>[2x]TDTTLPPDDSLDRIEPVDIEQEMQRSYIDYAMSVIVGRALPEVRDGLKPVHRRVLYAMFDSGFRPDRSHAKSARSVAETMGNYHPHGDSSIYDSLVRMAQPWSLRYPLVDGQGNFGSPGNDPPAAMRYTEARLTPLAMEMLREIDEETVDFIPNYDGRVQEPTVLPSRFPNLLANGSGGIAVGMATNIPPHNLRELADAVFWALENHDADEEETLAAVMGRVKGPDFPTAGLIVGSQGTADAYKTGRGSIRMRGVVEVEEDSRGRTSLVITELPYQVNHDNFITSIAEQVRDGKLAGISNIEDQSSDRVGLRIVIEIKRDAVAKVVINNLYKHTQLQTSFGANMLAIVDGVPRTLRLDQLIRYYVDHQLDVIVRRTTYRLRKANERAHILRGLVKALDAL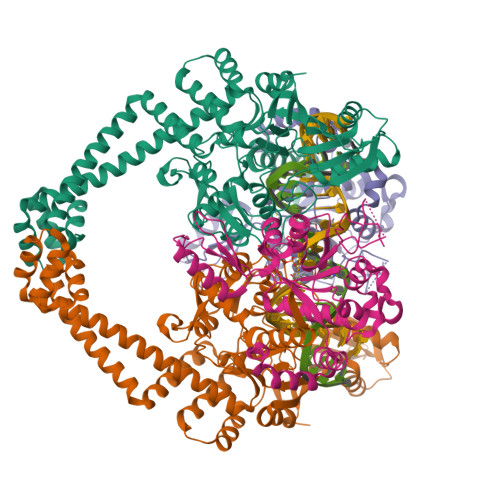DEVIALIRASETVDIARAGLIELLDIDEIQAQAILDMQLRRLAALERQRIIDDLAKIEAEIADLEDILAKPERQRGIVRDELAEIVDRHGDDRRTRIIAIGSG;>SNALVRRKSATDIGGLPGKLADCRSTDPRKSELYVVEGDSAGGSAKSGRDSMFQAILPLRGKIINVEKARIDRVLKNTEVQAIITALGTGIHDEFDIGKLRYHKIVLMADADVDGQHISTLLLTLLFRFMRPLIENGHVFLAQPPLYKLKWQRSDPEFAYSDRERDGLLEAGLKAGKKINKEDGIQRYKGLGEMDAKELWETTMDPSVRVLRQVTLDDAAAADELFSILMGEDVDARRSFITRNAKDVRFLDV[2x]>MLPKDKLNPPTPSIYLENKRDAFFPPLHQFCTNPKNPVTVIRGLAGALKLDLGLFSTKTLVEANNEHMVEVRTQLLQPADENWDPTGTKKIWRCESNRSHTTIAKYAQYQASSFQESLREENEKRTQHKDHSDNESTSSENSGRRRKGPFKTIKFGTNIDLSDNKKWKLQLHELTKLPAFARVVSAGNLLTHVGHTILGMNTVQLYMKVPGSRTPGHQENNNFCSVNINIGPGDCEWFVVPEDYWGVLNDFCEKNNLNFLMSSWWPNLEDLYEANVPVYRFIQRPGDLVWINAGTVHWVQAVGWCNNIAWNVGPLTACQYKLAVERYEWNKLKSVKSPVPMVHLSW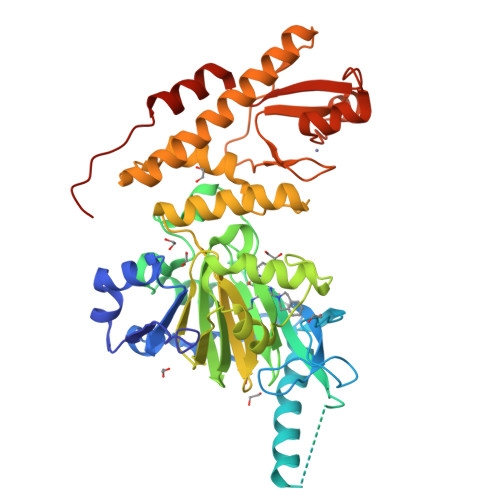NMARNIKVSDPKLFEMIKYCLLKILKQYQTLREALVAAGKEVIWHGRTNDEPAHYCSICEVEVFNLLFVTNESNTQKTYIVHCHDCARKTSKSLENFVVLEQYKMEDLIQVYDQFTLALSLSSSSAENLYFQ[2x]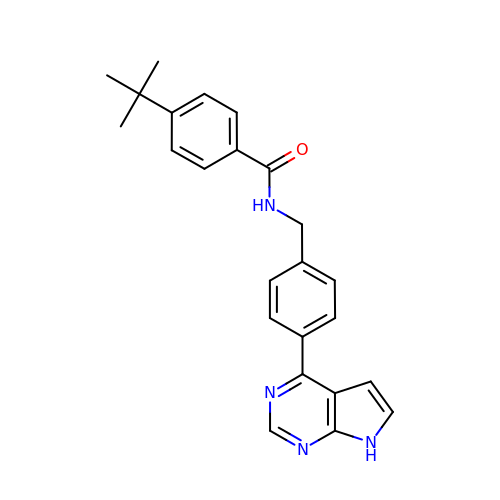4-~{tert}-butyl-~{N}-[[4-(7~{H}-pyrrolo[2,3-d]pyrimidin-4-yl)phenyl]methyl]benzamide | C24 H24 N4 O | ODLDMAFDYHTWSE-UHFFFAOYSA-N>MTNIAKAQPKLYVMDNGRMRMDKNWMIAMHNPATIANPNAPTEFIEFPIYTVLIDHPEGKILFDTSCNPDSMGAQGRWGEATQSMFPWTASEECYLHNRLEQLKVRPEDIKFVIASHLHLDHAGCLEMFTNATIIVHEDEFSGALQTYARNQTEGAYIWGDIDAWIKNNLNWRTIKRDEDNIVLAEGIKILNFGSGHAWGMLGLHVQLPEKGGIILASDAVYSAESYGPPIKPPGIIYDSLGFVRSVEKIKRIAKETNSEVWFGHDSEQFKRFRKSTEGYYE[3x]

AaL (WP_021296945.1) is a lactonase isolated from the acidophilic, moderately thermostable bacterium Alicyclobacillus acidoterrestris. The quorum quenching lactonase AaL from the thermoacidophilic bacterium Alicyclobacillus acidoterrestris exhibits a very broad substrate range, being capable of hydrolyzing short and long chain AHLs with high proficiencies. AaL possesses a bi-metallic active site center. We show that AaL is capable of degrading δ-lactones and γ-lactones with high catalytic proficiency (>104 M−1 s−1) and shows some weak, promiscuous phosphotriesterase activity on the insecticide-derivated paraoxon. The crystal structure of AaL reveals a unique hydrophobic patch which could relate to its high specificity, and highlights a flexible active site loop which may be involved in substrate binding.

Examination of one of the obtained AaL structure reveals the presence of a tetrahedral molecule in the active site, as clearly illustrated by the electronic density. Similarly to what was observed in the AiiB structure, this density was attributed to a phosphate anion. In this structure, the α-metal is bridged with H118, H120, H198, D220 and two phosphate oxygen atoms, while the β-metal is bound to H123, H266, D122, D220 and two oxygen atoms from the phosphate anion. With the bound phosphate, the bridging water molecule is not present in the metal coordination. Interestingly, the phosphate-bound AaL and AiiB structures differ in the way they coordinate the anion. However, in the case of AaL, the corresponding residue, a leucine, does not interact with the bound anion. In fact, metal coordination is affected and the distance between both metal cations varies greatly between the two enzymes (3.5 Å and 4.2 Å in AaL and AiiB, respectively, for the two phosphate-bound structures).> FTPX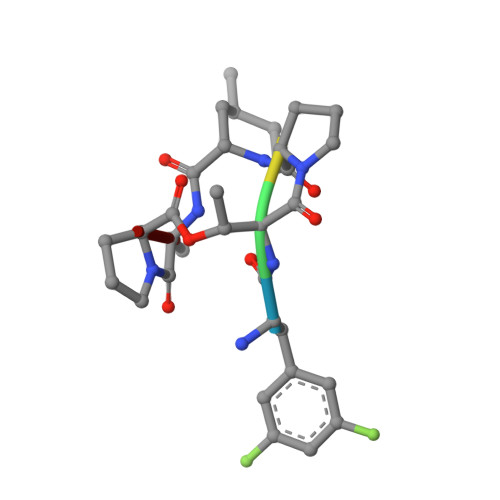AP(S)-2-HYDROXYPROPYLPHOSPHONIC ACID | C3 H9 O4 P 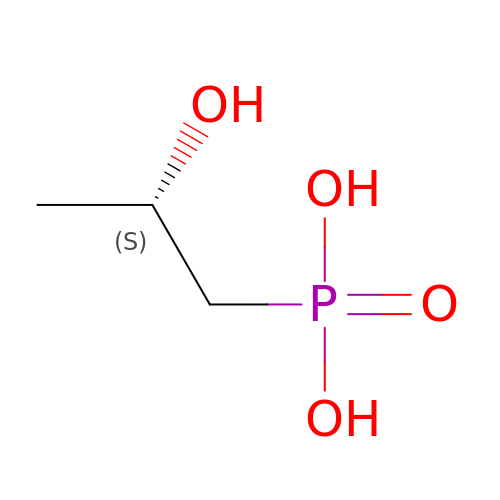| ZFVCONUOLQASEW-VKHMYHEASA-N> GSITTL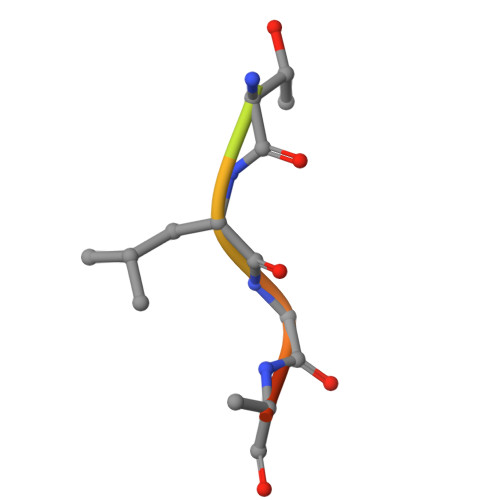GKFG4-hydroxybutyl trihydrogen 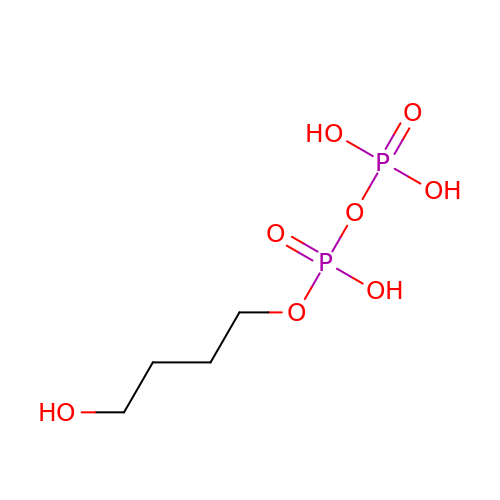diphosphate | C4 H12 O8 P2 | OLLDOFHGCGXIPA-UHFFFAOYSA-N>MQNITQSWFVQGMIWATTDAWLKGWDERNGGNLTLRLDDADIAPYHDNFHQQPRYIPLSQPMPLLANTPFIVTGSGKFFRNVQLDPAANLGIVKVDSDGAGYHI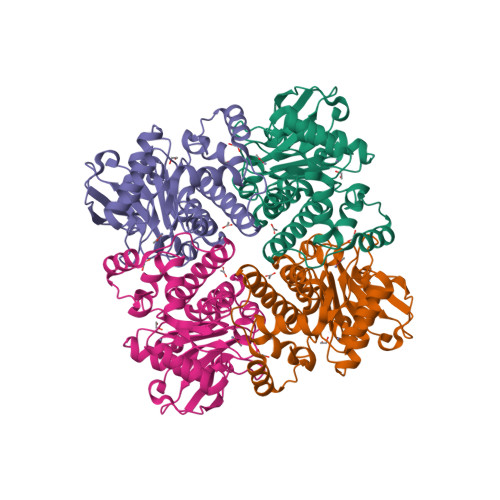LWGLTNEAVPTSELPAHFLSHCERIKATNGKDRVIMHCHATNLIALTYVLENDTAVFTRQLWEGSTECLVVFPDGVGILPWMVPGTDEIGQATAQEMQKHSLVLWPFHGVFGSGPTLDETFGLIDTAEKSAQVLVKVYSMGGMKQTISREELIALGKRFGVTPLASALAL[2x]>MESTLGWSVQDWLSFHSKSTPTKSLELLENLLKSQKPAPEDPAWISLIPVEDLHHQWNILQSKSNKEELPLYGVPIAVKDNIDYKGLPTTAACPSYLYQPTRDSYVVELLRDAGAVVIGKTNLDQFATGLVGTRSPYGKTPCVFNDKYVSGGSSAGSASVVGRGIVPLSLGTDTAGSGRVPAALNNLIGLKPTKGAFSCRGVVPACKSLDCVSVFALNLSDAEIAFKVMNKPDLLEDEYSREFPKNPISQYPKDLTIAIPKEVPWFGETENPKLYTKAVASLKNTGAKIVVVDFEPLLELARCLYEGAWVAERYCATRDFLATNPPESSLDETVVNIIKGAVKFDAADAFKFEYKRQGILQKVNLLLKDIDVLCVPTCPLNPKLEEVAQEPVLVNSRQGTWTNFVNLADLAALAVPSGFRSDGLPNGITLIGKKFSDYALLDLAKRFFSVAFPNNSRTYGKFVDRRITVEDELDGPSKDTLNGVKLAVVGAHLKGLPLHWQLQKCNATYLSSPKTSNNYKLYALPKVGPVLKPGLRRVNDGTGSQIQLEVYSVPYDRFGDFIAMVPEPLGIGSVELESGEWVKSFICEEFGYTQQGTVDITKFGGFKPYIEHIQVTEAQKKKPFETVLIANRGEIAVRIMKTLKRMGIKSVAVYSDPDKYSQHVTDADFSVALHGRTAAETYLDIDKIINAAKKTGAQAIIPGYGFLSENADFSDRCSQENIVFVGPSGDAIRKLGLKHSAREIAERAKVPLVPGSGLIKDAKEAKEVAKKLEYPVMVKSTAGGGGIGLQKVDSEDDIERVFETVQHQGKSYFGDAGVFMERFVNNARHVEIQMMGDGFGKAIAIGERDCSLQRRNQKVIEETPAPNLPEATRAKMRAASERLGSLLKYKCAGTVEFIYDEQRDEFYFLEVNARLQVEHPITEMVTGLDLVEWMLRIAANDSPDFDNTKIEVSGASIEARLYAENPVKDFRPSPGQLTSVSFPSWARVDTWVKKGTNVSAEYDPTLAKIIVHGKDRNDAIMKLNQALNETAVYGCITNIDYLRSIASSKMFKEAKVATKVLDSFDYKPCAFEVLAPGANTSVQDYPGRTGYWRIGVPPSGPMDSYSFRLANRVVGNNSKSPALEITLNGPKLLFHTETVIAVSGGTVSCTLNDAQIAQNEPIEVKRGDILSVGKVTVGCRAYLSIRGGIDVPEYLGSRSTFAMGNMGGYNGRILKLGDVLFLNQPELSVSSLPAPDFEPQAAPKSLLPTLSTNKDWKIGVTCGPHGSIDLFKEEYIEQFFNDKWKVHYNSNRFGVRLIGPKPKWARSDGGEAGLHPSNAHDYVYSLGAINFTGDEPVIITCDGPSLGGFVCQAVVAEAELWKVGQLTPGDTIQFVPLSYGVARQLKESQDKSIDNFEEGSLLELSDDKILPKYENPILAVLPKKSDLSPKVTYRQAGDRYILVEYGELEFDLNICYRINRLIHQVERHQTVGIVEMSQGVRSVLIEFDGSKINQKALLKCLIAYESEIQFDKNWNVKSKIFKLPMAFEDSKTLDCVTRYRETIRSEAPWLPNNVDFIADVNDIDRNDVKNMLYSAKFMVLGLGDVFLGSPCAVPLDPRHRYLGTKYNPSRTYTARGVVGIGGMYMCIYNAEGSPGGYQLVGRTITAWDKLVIGDHPIDHPWLLTPFDQVEFYPVTEEELEVIIEDNDNGKFKIDVEESIFDHKEYLAWINENIDSIVAFQEAQGGEKADEFARLIQVANAELKKSGDDKPQDVEEYPDDAELLYSEYTGRFWKPVAAVGDHVEAGDGVIIIEAMKTEMVVGATKSGKVYKILHKNGDMVEAGDLVAVIV[4x]

The first step of their urea utilization is the conversion of urea to ammonium, which is catalyzed by two distinct enzymes, urease and urea amidolyase (UA). UA is composed of urea carboxylase (UC) and allophanate hydrolase (AH) domains. UC converts urea to allophanate, and AH subsequently converts it to ammonium. Biotin is covalently linked to its biotin-carboxyl carrier protein (BCCP) domain. Its biotin carboxylase (BC) and carboxyltransferase (CT) domains catalyze sequential reactions in urea caboxylation.

We present here crystal structure of Kluyveromyces lactis UA (KlUA) at 6.5 Å resolution. We speculated that the mobility of the BCCP domain prevented its crystallization, and hence removed it. This variant (residues 1–1741, KlUAΔBCCP) crystallized with the vapor diffusion method. Despite extensive efforts, the best crystals only diffract to 6–7 Å resolution at the Shanghai Synchrotron Radiation Facility. They belong to space group P212121 and contain four copies of KlUAΔBCCP in the asymmetric unit. In the crystal the four KlUAΔBCCP polypeptides are organized into two very similar dimers. The structure of the dimer resembles the letter ‘m’, with the AH domains at the center, sandwiched by the UC domains on both sides. In the KlUA dimer, the interactions between the monomers are located at two interfaces. One is between the AH domains, which form a dimer identical with the isolated KlAH. The other is between the UC CT domain and the AH N domain from the other polypeptide. This interface is mainly contributed by helices αH and αI in the UC CT domain, and helix α3 in the AH N domain, burying 1000 Å2 of surface area. In the KlUAΔBCCP structure, these active sites are located more than 70 Å apart.> NGAAKIITIVPLVNDLDPLDILYKLLKCADDEGIMVQEVDSKRIFNVHIKKFKSNLKIIIPDMTNFLNILDCAKVADFVVFGLSGVQEVDEEFGEQIIRALELQGIASYIGVISNLSAVHEKEKFQLDVKQSLESYFKHFFPSEERVYNLEKNSDALNVLRTLCQRLPRSINWRDNRGYVVADFVDFVETSPDSGDLVIEGTVRGIGFNANRLVHIPDFGDFQLNKIEKISESSQKRKIIKEKATDSLSLELDLQTVFESNMNRDTLDEYAPEGTEDWSDYDEDFEYDGLTTARYDDHGFLPGREQTSKKAAVPKGTSDYQAKWYLDDVIDANEEEEAEQTNGKDETMMEIDDEMMVEQDNEEVAGDEEYDIEDNEGFEELSPEEEERQLREFRDMEKEDREFPDEIELEPSESAIERLKRYRGLKNLYNCDWQVDEKDPSSPAEWKRLLRIGNYKNTKNRIIKETKNEAQAIAGDRIRMFIRFPKFLLEKIQDPKQLLFAVYGLLLHEHKNAVVNFSLQRWEQYDKPVPSQEPIVVQYGVRRYTIQPLFSQGSNSPNNVHKYERFLHPDTVSVATCIAPVDFTQSPAIFFKPSPTDAKNIELIGHGTFLNADHSRILAKRAILTGHPFRFHKTVVTVRYMFFRPEDVEWFKSIPLFTKSGRSGFIKESLGTHGYFKATFDGKLSAQDVVAMSLYKRMWPMPSLPWNGM

The 5' region of pre-rRNA that consists of the 5' external transcribed spacer (5' ETS), 18S rRNA and the internal transcribed spacer 1 (ITS1) is co-transcriptionally packed into a terminal ball of ~40 nm in size. These particles represent the earliest assembly intermediates of 40S and are known as the 90S pre-ribosome or the SSU processome. Within 90S, the pre-rRNA is cleaved at sites A0 and A1 in the 5' ETS and site A2 in the ITS1, yielding a 20S pre-rRNA intermediate. The fully assembled 90S contains an unprocessed pre-18S rRNA, U3 snoRNA, approximately 51 assembly factors and 18 r-proteins with a molecular mass of 5.0 megadaltons.

Bms1 is a GTPase and associates with Rcl1. The binding site of Bms1 overlaps significantly with that of Tsr1, suggesting that Bms1 is replaced by Tsr1 during the transition of 90S to pre-40S.Human RON (Recepteur d’Origine Nantais) receptor tyrosine kinase is the specific cell-surface receptor for Macrophage Stimulating Protein (MSP), a serum growth factor also known as the Hepatocyte Growth Factor-like protein (HGFL). RON, encoded by the MST1R gene, is a member of the Class VI receptor tyrosine kinase family (EC:2.7.10.1) along with the proto-oncogene Met receptor tyrosine kinase (Met). RON comprises an extracellular ligand binding domain (ectodomain), a single pass trans-membrane segment and a cytoplasmic tyrosine kinase domain. The ectodomain can be subdivided into the N-terminal semaphorin (Sema) domain, a small cysteine-rich Plexins-Semaphorins-Integrins (PSI) motif, and four Immunoglobulins-Plexins-Transcription factor (IPT) domains.

Here, we report the crystal structure of RON Sema-PSI domains at 1.85 Å. Overall, the RON Sema-PSI model contains amino acids Val42–Pro568 except for nine Sema residues encompassing the disordered thrombin cleavage site (Leu306–Gly314) and four loop residues (Asp355–Pro358). Of the four predicted RON Sema N-glycosylation sites (Asn66, Asn419, Asn458, and Asn488), only the Asn488 N-glycan was visible in the electron density map, consistent with a branched biantennary oligosaccharide Manα(1,3)Manβ(1,4)GlcNAcβ(1,4)GlcNAc. The RON Sema domain adopts the seven-bladed β-propeller fold, found in Met, semaphorins and plexin receptors. In RON, the 62-residue insertion (Pro370–Ser432) is located between β-strands 5C and 4E, and it forms a 16-residue helix (αEX1), followed by a long loop that packs tightly against the outermost 4E. The PSI motifs of RON and Met adopt a cysteine-knot fold consisting of two small antiparallel β-sheets and four short α-helices. The interdomain contact area between the RON Sema and PSI domains embeds ∼385 Å2 surface area. In all, the alternate disulfide bonding patterns in the 1D–2A loop and the extrusion regions of RON and Met Sema domains define specificity determinants, which allow RON and Met receptors to interact exclusively with either MSP or HGF, respectively. RON intermolecular interactions generated by the crystal packing reveal a potential mode of ligand-independent dimerization, mediated by the Sema domain. This is the most extensive crystallographic related RON Sema-Sema interface with ∼960 Å2 embedded surface area, a rather large interface for typical crystal contacts.

> VKYVVPSFSAGGLVQAMVTYEGDRNESAVFVAIRNRLHVLGPDLKSVQSLATGPAGDPGCQTCAACGPGPHGPPGDTDTKVLVLDPALPALVSCGSSLQGRCFLHDLEPQGTAVHLAAPACLFSAHHNRPDDCPDCVASPLGTRVTVVEQGQASYFYVASSLDAAVAASFSPRSVSIRRLKADASGFAPGFVALSVLPKHLVSYSIEYVHSFHTGAFVYFLTVQPASVTDDPSALHTRLARLSATEPELGDYRELVLDCRFAPKLVPRGSPEGGQPYPVLQVAHSAPVGAQLATELSIAEGQEVLFGVFVTGKDGGPGVGPNSVVCAFPIDLLDTLIDEGVERCCESPVHPGLRRGLDFFQSPSFCPNPPGLEALSPNTSCRHFPLLVSSSFSRVDLFNGLLGPVQVTALYVTRLDNVTVAHMGTMDGRILQVELVRSLNYLLYVSNFSLGDSGQPVQRDVSRLGDHLLFASGDQVFQVPIQGPGCRHFLTCGRCLRAWHFMGCGWCGNMCGQQKECPGSWQQDHCP> MFSRPGLPVEYLQVPSASMGRDIKVQFQGGGPHAVYLLDGLRAQDDYNGWDINTPAFEEYYQSGLSVIMPVGGQSSFYTDWYQPSQSNGQNYTYKWETFLTREMPAWLQANKGVSPTGNAAVGLSMSGGSALILAAYYPQQFPYAASLSGFLNPSESWWPTLIGLAMNDSGGYNANSMWGPSSDPAWKRNDPMVQIPRLVANNTRIWVYCGN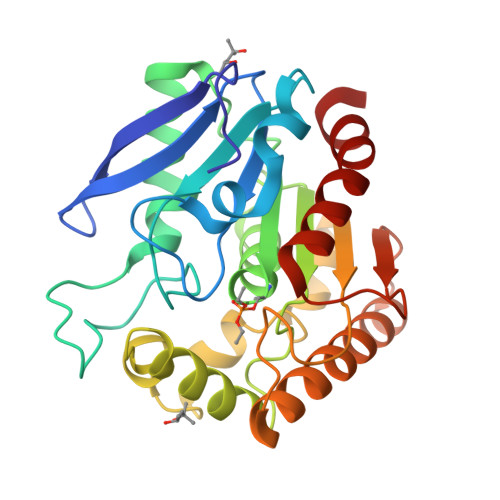GTPSDLGGDNIPAKFLEGLTLRTNQTFRDTYAADGGRNGVFNFPPNGTHSWPYWNEQLVAMKADIQHVLNG> HPKLVSSTPAEGSEGAAPAKIELHFSENLVTQFSGAKLVMTAMPGMEHSPMAVKAAVSGGGDPKTMVITPASPLTAGTYKVDWRAVSSDTHPITGSVTFK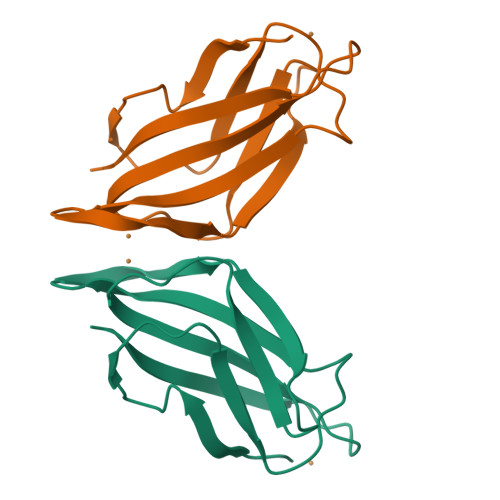VK>[2x]MDITEERLHYQVGQRALIQ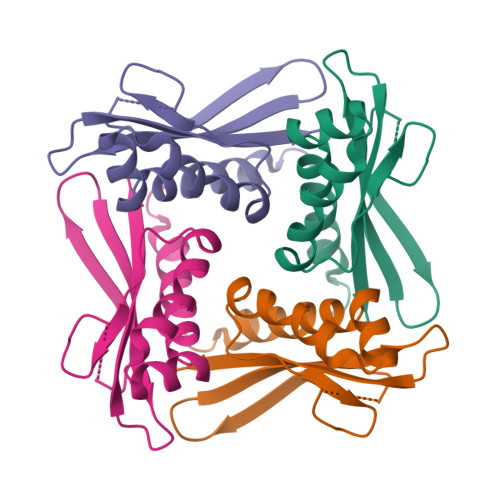AMQISAMPELVEAVQKRDLARIKALIDPMRSFSDATYITVGDASGQRLYHVNPDEIGKSMEGGDSDEALINAKSYVSVRKGSLGSSLRGKSPIQDATGKVIGIVSVGYTIEQLE> GSTYDALRRQLIPSFDLLYGSAVSVVAMSVPATARILDLGAGTGLLGAALRERLPDAELLLQDRSQAMLEQARQRFADDDQVAIRVADHLDELPAGPFDAVVSALSIHHLEHQDKQDLFTRIRKILRPGGIFVNVEQVLAPTSELEKMYDRQHEAHVLASDTPAEEWAAGRERMKHDIPIDVETQIQWLRDAGFTTADCLAKDWRFATYAGWNGS

Here, we characterize the O-methyltransferases BelI and CysG, which catalyze the initial step of β-lactone formation. Employing techniques such as crystallography, computational analysis, mutagenesis, and activity assays, we identified a His-His-Asp (HHD) motif in the active sites of the two enzymes, which is crucial for binding a catalytically active calcium ion. As expected, BelI as well as CysGΔN16 adopt the class I methyltransferase Rossmann fold, characterized by a core domain of a seven-stranded β-sheet flanked by α-helices. The HHD-motif enables regiospecific C1-carboxy group methylation of their respective malic substrates.

The crystal structures of CysGΔN16 in complex with S-adenosylhomocysteine (SAH) and BelI bound to SAM were solved at 1.5 Å and 1.95 Å, respectively. Intriguingly, the crystal structures of CysGΔN16 and BelI revealed a His122-His123-Asp191 (HHD) motif with additional strong positive electron density, indicative of a divalent metal ion. The absence of anomalous signals in X-ray fluorescence experiments conducted with the crystals suggests calcium or magnesium as likely candidates. Notably, the complex depicts octahedral metal coordination with bond lengths between 2.0 and 2.4 Å and bond angles, which are consistent with the binding profile of calcium (Ca2+). Specifically, the terminal carboxyl and amino groups of SAH/SAM are forming hydrogen bonds with Tyr33, Gly54, and residue 118. The ribose unit is coordinated via Asp77, while the adenine portion is stabilized by Asp102, residue 103, and cation-π interactions with Arg78. Notably, the N-terminally truncated CysGΔN16 variant was active with metal ions available but inactive in the presence of EDTA.>[2x]GLSRGPSPISLSAQESWPVAAAITEYINAYFRGGEHNRCLVKITGDLTMSFPAGITRIFTANPNAPVLSFRLVNISRVDHFLPN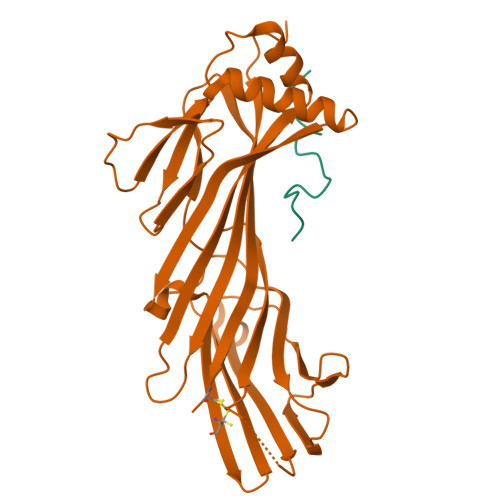QKLLYSDPSQSDPDTKDFWFNMQALTLHLQREAELNPQASYYNVALLKYQASSQDPSRAPLLLSAECQRSGTVTRVSLDYHCCPATAPATQLTSVQVLLPLDHSATDLQCQPPAAWNAEERRLLWKLANLSPTNHSKGSGTLCASWQCLEVPRGPAPSLAVQFVGSGASLSGLDVELVGSRYRMSLVKKRFATGKYMAGCSL;>TNLDFFQSDPFVGSDPFKDDPFGGAGA[2x]> SFDCGKPQVEPKKCPGRVVGGCVAHPHSWPWQVSLRTR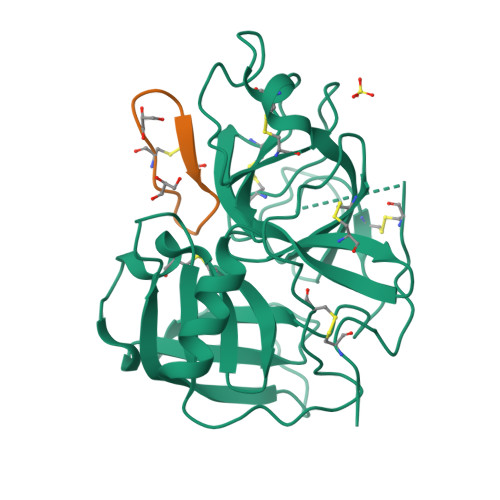FGMHFCGGTLISPEWVLTAAHCLEKSPRPSSYKVILGAHQEVNLEPHVQEIEVSRLFLEPTRKDIALLKLSSPAVITDKVIPACLPSPNYVVADRTECFITGWGETQGTFGAGLLKEAQLPVIENKVCNRYEFLNGRVQSTELCAGHLAGGTDSCQGDSGGPLVCFEKDKYILQGVTSWGLGCARPNKPGVYVRVSRFVTWIEGVMRNN;> GRCTKSRPPICFPD>[2x]TQKPSL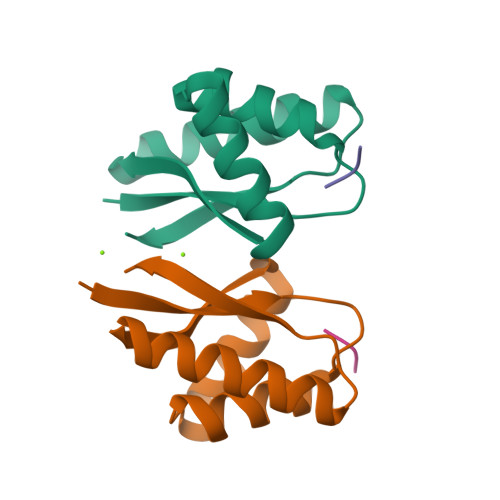YRVLILNDDYTPAEFVVYVLERFFNKSREDATRIMLHVHQNGVGVCGVYTYEVAETKVAQVIDSARRHQHPLQCTMEKD;>[2x]WLFVQRDSKE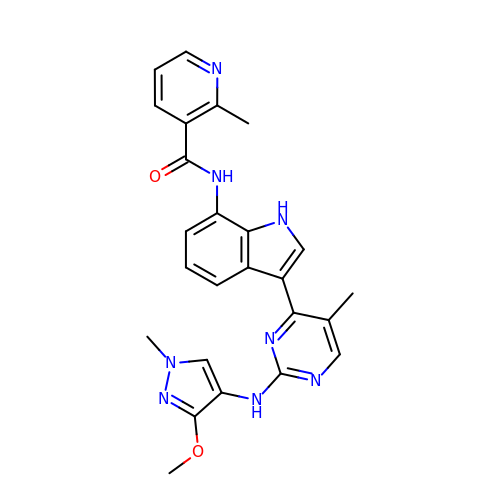~{N}-[3-[2-[(3-methoxy-1-methyl-pyrazol-4-yl)amino]-5-methyl-pyrimidin-4-yl]-1~{H}-indol-7-yl]-2-methyl-pyridine-3-carboxamide | C25 H24 N8 O2 | VVOKUJIAOSWPTI-UHFFFAOYSA-N>[4x]LASMWELTILHTNDVHSRLEQTSEDSSKCVDA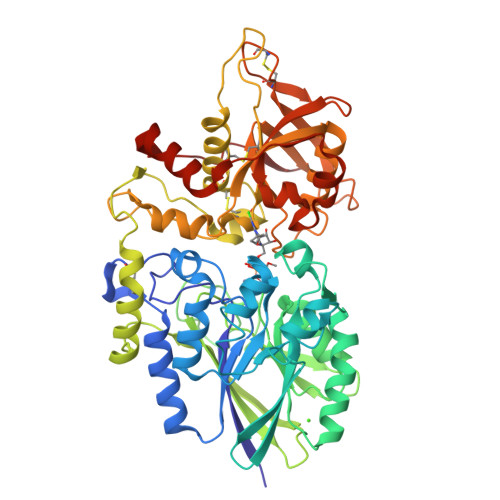SRCMGGVARLFTKVQQIRRAEPNVLLLDAGDQYQGTIWFTVYKGAEVAHFMNALRYDAMALGNHEFDNGVEGLIEPLLKEAKFPILSANIKAKGPLASQISGLYLPYKVLPVGDEVVGIVGYTSKETPFLSNPGTNLVFEDEITALQPEVDKLKTLNVNKIIALGHSGFEMDKLIAQKVRGVDVVVGGHSNTFLYTGNPPSKEVPAGKYPFIVTSDDGRKVPVVQAYAFGKYLGYLKIEFDERGNVISSHGNPILLNSSIPEDPSIKADINKWRIKLDDYSTQELGKTIVYLDGSSQSCRFRECNMGNLICDAMINNNLRHTDEMFWNHVSMCILNGGGIRSPIDERNDGTITWENLAAVLPFGGTFDLVQLKGSTLKKAFEHSVHRYGQSTGEFLQVGGIHVVYDLSRKPGDRVVKLDVLCTKCRVPSYDPLKMDEVYKVILPNFLANGGDGFQMIKDELLRHDSGDQDINVVSTYISKMKVIYPAVEGRIKFSHH>GAMASGKVVKFSYMWTINNFSFCREKMGEVIKSSTFSSGANDKLKWCLRVNPKGLDE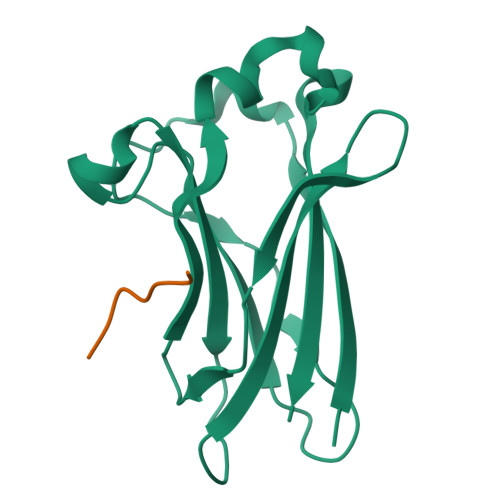ESKDYLSLYLLLVSCPKSEVRAKFKFSILNAKGEETKAMESQRAYRFVQGKDWGFKKFIRRDFLLDEANGLLPDDKLTLFCEVSVVQD[4x];>[4x]KADTTTPTT>[2x]MPERITLYTAKICPFAQRAEIALAEAKAEFTPFQIDLSNKPEWYAPKVNPASKVPA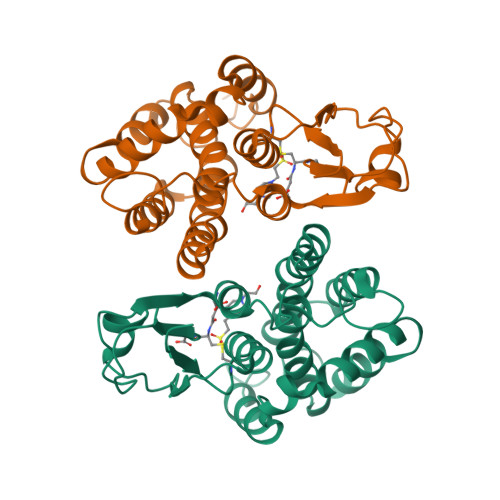IAYGGPEVPPDQPSPESVKLAESLVLVEFVADLFPNSGILSSDPVTRAQTRFFIEGVSSKLIPAWYAYFLRGASVDDLYTAAEYVQSLLPAEGFAVGKFSAADIAIAPFLARARVSLVNEIGKYPEGDGKKVWAALTSGKFARLGKYAEDLFARESFSSTFDEDYVTKAFSARFADLRSKHHHHHH>[2x]GPGSMSSNSLKFGTSGLRGLAVELNGLPAYAYTMAFVQMLAAKGQLQKGDKVFVGRDLRPSSPDIAALAMGAIEDAGFTPVNCGVLPTPALSYYAMGAKAPSIMVTGSHIPDDRNGLKFYRRDGEIDKDDEAAISAAYRKLPAILAARKHVGSTETDAALQAYADRYAGFLGKGSLNGLRVGVYQHSSVARDLLMYLLTTLGVEPVALGRSDIFVP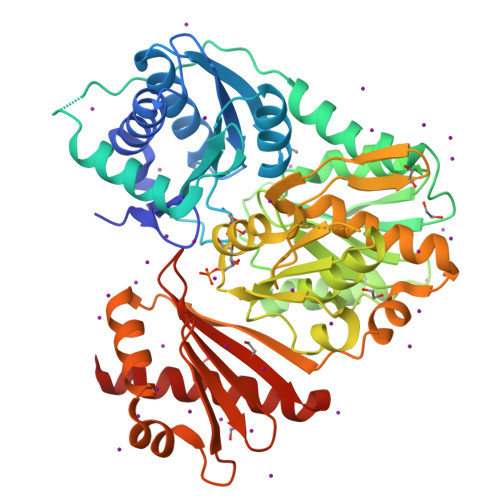VDTEALRPEDIALLAQWGKSDRLDAIVSTDGDADRPLIADEHGQFVRGDLAGAITATWVGADTLVTPVTSNTALESRFPKVLRTRVGSPYVIASMAQVSTGNSGPVIGFEANGGVLLGSTVERNGRSLTALPTRDALLPILACLATVHEKKTPLSTIARSYGFRVALSDRLQNIPQEASTAFLALLEDADKRASLFPAGDAIVRVETIDGVKLFFQSGNAVHYRASGNAPELRCYVESSDDTQAAKLQALGLEIARKALKDATRP>[4x]SKETKPLPDYVAWKDADALIVHSDKTLETKRSEFGTSIITPEEKLYIRNNVNTPPESILADRDGWKVEISGVKEPRTLTVAELKTLGLVTAATVLQCSGNGRKYFKDQLTGDQKMSGTPWTVGAAGCVIWSGVPLKAVVDALGGPAEGARFITGTGGEELPAGLDPKLLVVERSVPISNLDNVILAWEMNGRPLSLAHGGPLRMVV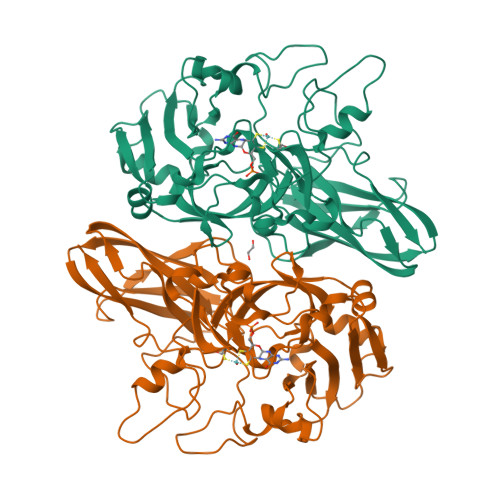PGYSGVNNIKYVKAVAMTEVETDAKIQKTSYRVHALGEKGSPDQPSVWEQPVKSWITTPHEAAKAGQVQIAGVAFGGMNACKSVEVSVDGGQTWQEAEFIGPDLGRFAWRVFALSADLARGTYTLVSRATDTEGNVQPEETEMNGAGYGHNGWRAPAVKLTVA>GSHMLADKVKLSAKEILEKEFKTGVRGYKQEDVDKFLDMIIKDYETFHQEIEELQQENLQLKKQLE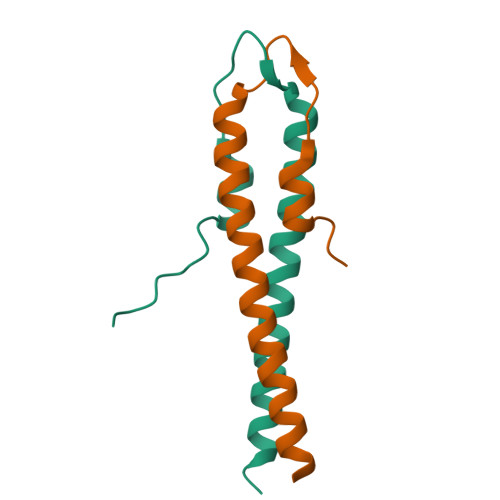EASKK[4x]>MGHHHHHHEFMTSRPSSDQTWQPIDGRVALIAPASAIATEVLEATLRQLEVHGVDYHLGRHVEARYRYLAGTVEQRLEDLHNAFDMPDITAVWCLRGGYGCGQLLPGLDWGRLEAASPRPLIGFADISVLLSAFHRHGLPAIHGPVATGLGLSPLSAPREQQERLASLASVSRLLAGIDHELPVQHLGGHKQRVEGALIGGNLTALACMAGTLGGLHAPAGSILVLEDVGEPYYRLERSLWQLLESIDARQLGAICLGSFTDCPRKEV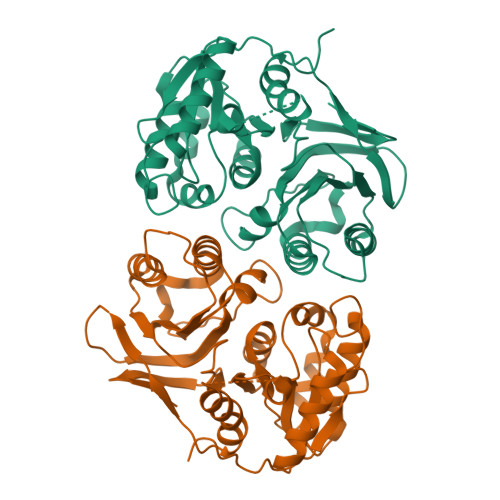AHSLERIFGEYAAAIEVPLYHHLPSGHGAQNRAWPYGKTAVLEGNRLRW[2x]>GMPRPKLKSDDEVLEAATVVLKRCGPIEFTLSGVAKEVGLSRAALIQRFTNRDTLLVRMMERGVEQVRHYLNAIPIGAGPQGLWEFLQVLVRSMNTRNDFSVNYLISWYELQVPELRTLAIQRNRAVVEGIRKRLPPGAPAAAELLLHSVIAGATMQWA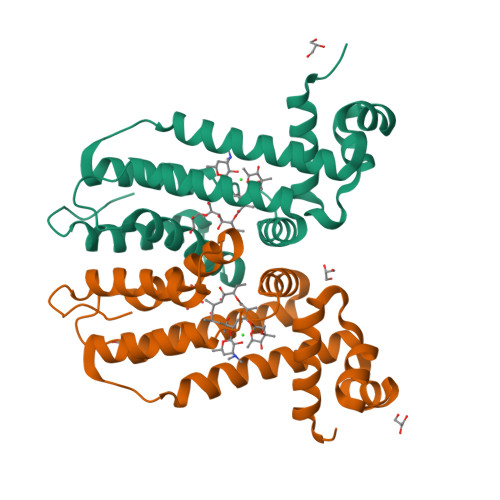VDPDGELADHVLAQIAAILCLMFPEHDDFQLLQAHA[2x]>[2x]VHHPPSYVAHLASDFGVRVFQQVAQASKDRNVVFSPYGVASVLAMLQLTTGGETQQQIQAAMGFKIDDKGMAPALRHLYKELMGPWNKDEISTTDAIFVQRDLKLVQGFMPHFFRLFRSTVKQVDFSEVERARFIINDWVKTHTKGMISHLLGTGAVDQLTRLVLVNALYFNGQWKTPFPDSSTHRRLFHKSDGSTVSVPMMAQTNK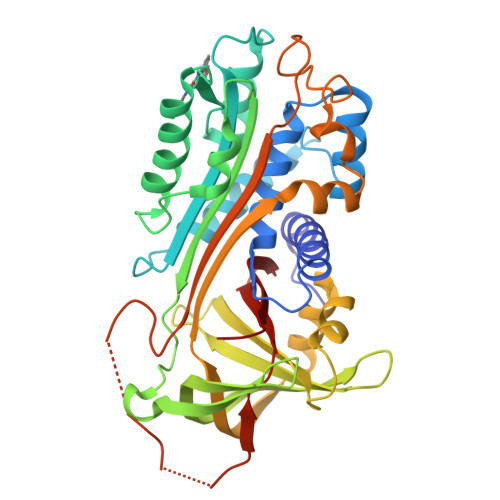FNYTEFTTPDGHYYDILELPYHGDTLSMFIAAPYEKEVPLSALTNILSAQLISHWKGNMTRLPRLLVLPKFSLETEVDLRKPLENLGMTDMFRPFQADFTSLSDQEPLHVALALQKVKIEVNESGTVASSSTAVIVSARMAPEEIIIDRPFLFVVRHNPTGTVLFMGQVMEP> MAQVQQLTPAQQAALRNQQAMAANLQARQIVLQQSYPVIQQVET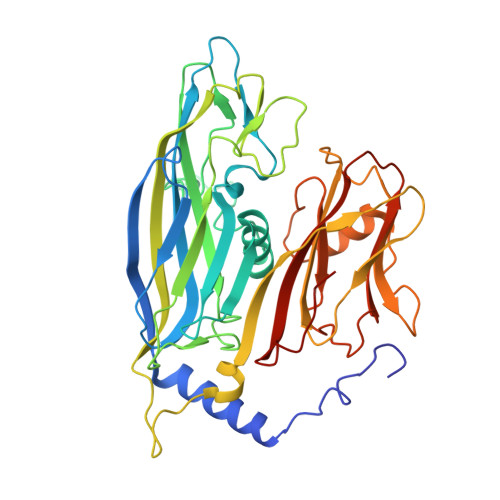QTFDPANRSVFDVTPANVGIVKGFLVKVTAAIKNNHATEAVALTDFGPANLVQRVIYYDPDNQRHTETSGWHLHFVNTAKQGAPFLSSMVTDSPIKYGDVMNVIDAPATIAAGATGELTMYYWVPLAYSETDLTGAVLANVPQSKQRLKLEFANNNTAFAAVGANPLEAIYQGAGAADCEFEEISYTVYQSYLDQLPVGQNGYILPLIDLSTLYNLENSAQAGLTPNVDFVVQYANLYRYLSTIAVFDNGGSFNAGTDINYLSQRTANFSDTRKLDPKTWAAQTRRRIATDFPKGVYYCDNRDKPIYTLQYGNVGFVVNPKTVNQNARLLMGYEYFTSRTELVNAGTISTT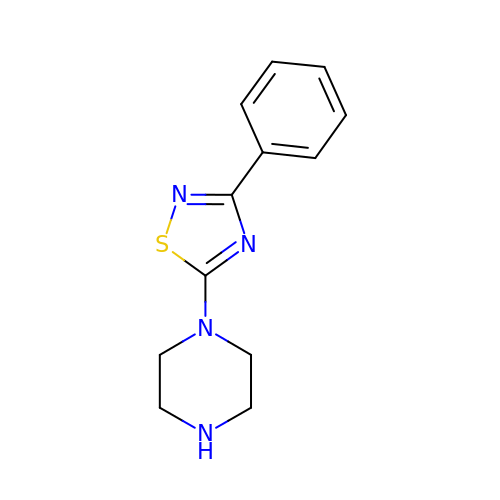1-(3-phenyl-1,2,4-thiadiazol-5-yl)piperazine | C12 H14 N4 S | UMFMHSLRNJBGKO-UHFFFAOYSA-N> MTHDNKLGVEAIKRGTV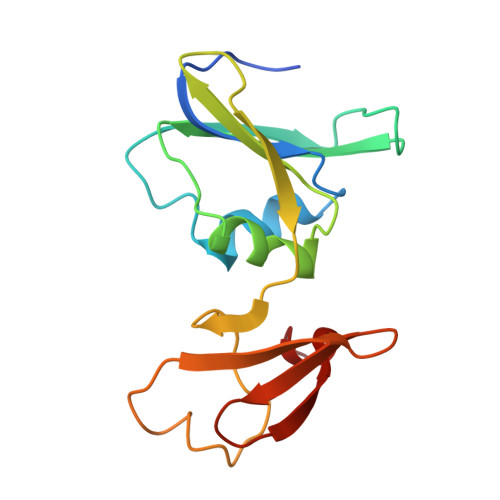IDHIPAQIGFKLLSLFKLTETDQRITIGLNLPSGEMGRKDLIKIENTFLSEDQVDQLALYAPQATVNRIDNYEVVGKSRPSLPERIDNVLVCPNSNCISHAEPVSSSFAVRKRANDIALKCKYCEKEFSHNVVLAN>[2x]MNHKVHHHHHHMKANQVQPLNKYPVVFVHGFLGLVGDNAPALYPNYWGGNKFKVIEELRKQGYNVHQASVSAFGSNYDRAVQLYYYIKGGRVDYGAAHAAKYGHERYGKTYKGIMPNWEPGKKVHLVGHAMGGQTIRLMEEF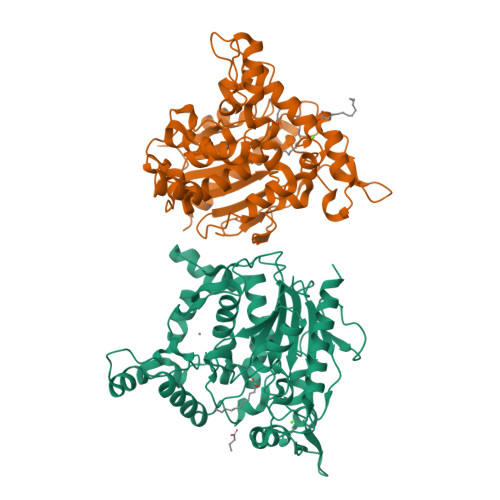LRNGNKEEIAYHQAHGGEISPLFTGGHNNMVASITTLATPHNGSQAADKFGNTEAVRKIMFALNRFMGNKYSNIDLGLTQWGFKQLPNESYIDYIKRVSKSKIWTSDDNAAYDLTLDGSAKLNNMTSMNPNITYTTYTGVSSHTGPLGYENPDLGTFFLMDTTSRIIGHDAREEWRKNDGVVPVISSLHPSNQPFVNVTNNEPATRRGIWQVKPILQGWDHVDFIGVDFLDFKRKGSELANFYIGIINDLLSVEATEGKGTQLKAS>[2x]GSLRGTTQKVNRIREITAMKTVEALQISAQLTQLHEVDMTRVAELRKKNKPAFIEKHGVNLTYLPFFVKAVVEA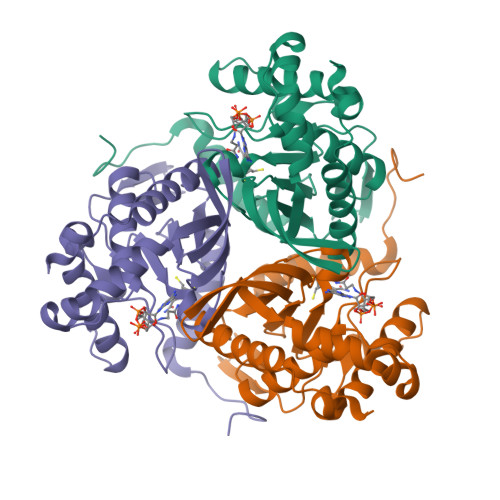LVSHPNVNASFNAKTKEMTYHSSVNLSIAVDTPAGLLTPVIHDAQDLSIPEIAKAIVDLADRSRNNKLKPNDLSGGTFTITNIGSEGALSDTPILVPPQAGILGTGAIVKRPVVITEDGIDSIAIRQMVFLPLTYDHQVVDGADAGRFLTTIKDRLETANFEGDLQL>NGEDAVPYSWSWQVSLQYEKDGAFHHTCGGSLIAPDWVVTAGHCISTSRTYQVVLGEYDRSVLEGSEQVIPINAGDLFVHPLWNSNCVACGNDIALVKLSRSAQLGDKVQLANLPPAGDILPNEAPCYISGWGRLYTGGPLPDKLQQALLPTVDYEHCSQWDWWGITVKKTMVCAGGDTRSGCNGDSGGPLNCPAADGSWQVHGVTSFVSAFGCNTIKK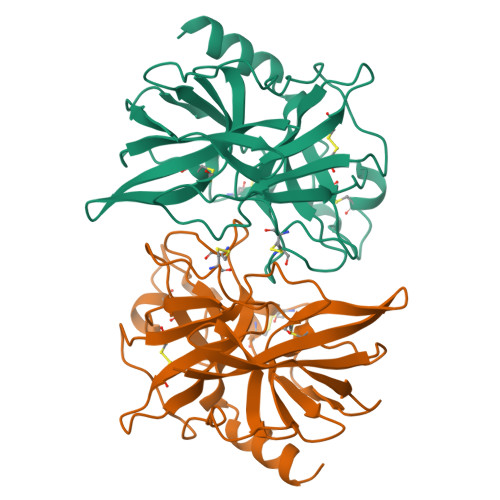PTVFTRVSAFIDWIDETIASN[2x]> MTRINLTLVSELADQHLMAEYRQLPRVFGAVRKHVANGKRVRDFKISPTFILGAGHVTFFYDKLEFLRKRQIELIAECLKRGFNIKDTTVQDISDIPQEFRGDYIPHEASIA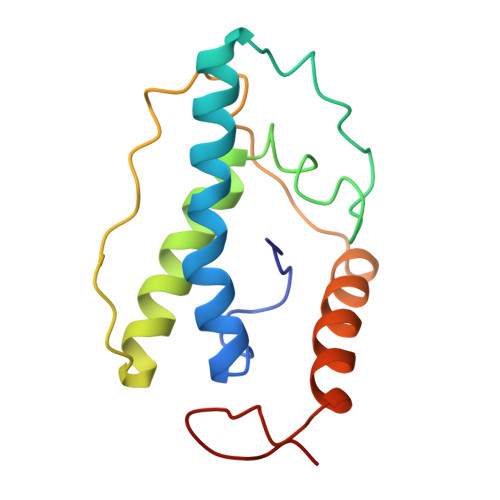ISQARLDEKIAQRPTWYKYYGKAIYA> ATDIRQVVDSTVEPLMQQQDIAGLSVAVIQNGKAQYFNYGVANKDSKQPITENTLFEIGSVSKTFTATLAGYALANGKLKLSDPASQYLPALRGDKFDHISLLNLGTYT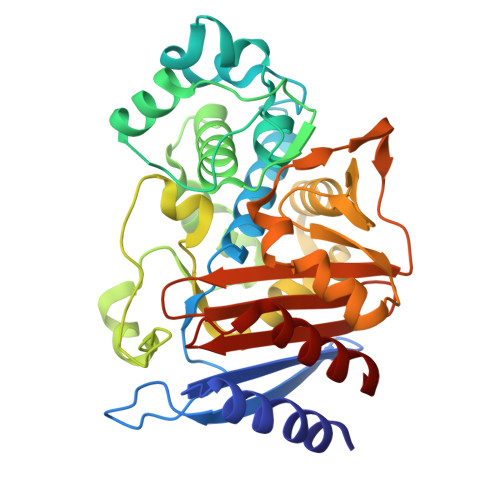AGGLPLQFPEESDNTGKMISYYQHWKPAFAPGTQRLYSNPSIGLFGHLAAQSLGQPFEKLMEQTVLPKLGLKHTFISVPETQMSLYAQGYDKAGKPVRVSPGALDAEAYGIKTSTSDLIHYVEVNMHPAKLEKPLQQAIAATHTGYYTVDGMTQGLGWEMYPYPIKVDALVEGNSTQMAMEPHKVNWLTPPQAAPLDTLVNKTGSTGGFGAYVAYVPSKGLGVVILANKNYPNAERVKAAHAILSAMDQ N-{4-[(R)-methylsulfinyl]butyl}thioformamide | C6 H13 N O S2 | 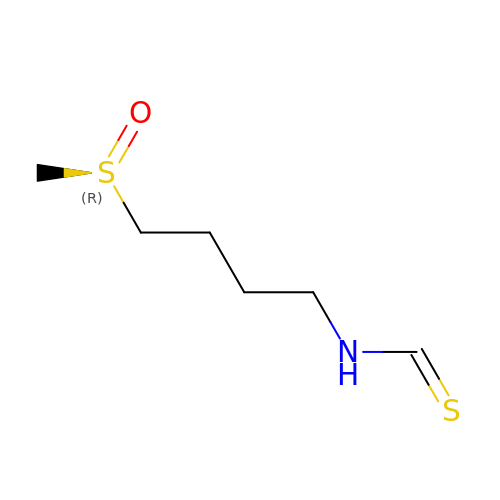ZWRKPZDQBQKJAE-SNVBAGLBSA-N(4~{S})-6-azanyl-4-[3-(2-cyanophenyl)-5-(trifluoromethyl)phenyl]-3-methyl-4-propan-2-yl-2~{H}-pyrano[2,3-c]pyrazole-5-carbonitrile 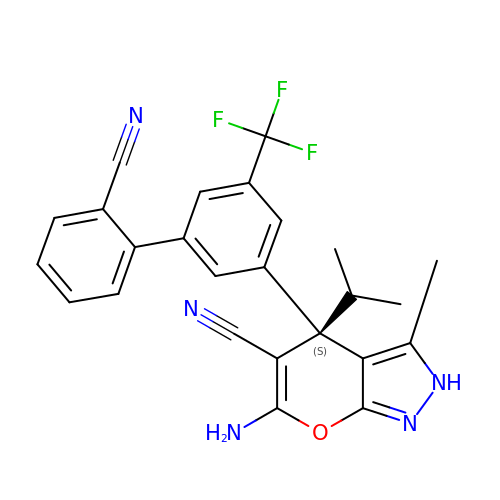| C25 H20 F3 N5 O | ZYSRKKYQJKRKDR-DEOSSOPVSA-N> STMEN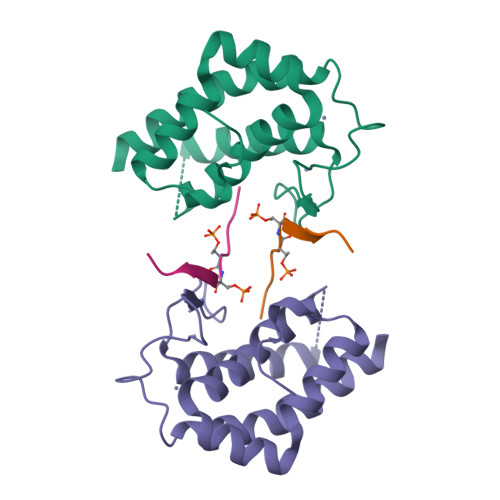IDKILEPPEGQDEGVWKYEHLRQFCLELNGLAVKLQSECHPDTCTQMTATEQWIFLCAAHKTPKECPAIDYTRHTLDGAACLLNSNKYFPSRVSIKESSVAKLGSVCRRIYRIFSHAYFHHRQIFDEYENETFLCHRFTKFVMKYNLMSKDNLIVPI;> THPEWSFTTVRKKPDP Soluble HMW1C-like N-glycosyltransferases (NGTs) catalyze the glycosylation of Asn residues in proteins, a process fundamental for bacterial autoaggregation, adhesion and pathogenicity. In contrast, NGTs are two-domain enzymes that consists of an N-terminal all-α domain (AAD) and a C-terminal catalytic domain that adopts a GT-B fold, as shown for Actinobacillus pleuropneumoniae NGT (ApNGT). We focused on AaNGT, an inverting GT that catalyzes the transfer of Glc from UDP-Glc to Asn residues in the consensus sequence Asn-X-Ser/Thr. The heart-shaped structure of AaNGT, either complexed to UDP-Gal/UDP-2F-Glc or UDP-peptide, shows the N-terminal AAD domain and C-terminal GT-B fold catalytic domain, which is composed of an N- and C-Rossman fold subdomains.

A surface representation of the ternary complex reveals that UDP is partly buried and mainly recognized by the C-Rossmann fold subdomain while the peptide is more solvent exposed and tethered mostly by the N-Rossmann fold subdomain and the AAD domain. The UDP pyrophosphate of the ternary complex (AaNGT + UDP + peptide) exhibits more interactions than in the binary complexes, with Thr519, Asn520, and Gly521 backbones, and Ser277, Thr437, Lys440, and Asn520 side chains contributing to this. Additionally, interactions with Arg280 are observed in the ternary complex. Therefore, these more extensive interactions of UDP with the enzyme could explain the higher affinity of UDP compared to the sugar nucleotides. Multiple hydrogen bond interactions are observed at the peptide binding site in the ternary complex (AaNGT-peptide-UDP). The structural data demonstrate that the key residues involved in recognition of the peptide are Arg177, His214, and Asp215 from the AAD domain. In summary, the structural analysis shows that NGT shares two critical and conserved residues among NGTs, Arg177 and Asp215, in the AAD domain that recognize Thr and likely Ser at the +2 position of the Asn0-X+1-Ser/Thr+2 sequence motif. CH-π interactions between the peptide and the protein were also observed, in particular those involving Trp4+1 and the methylene group of Gln468 (AaNGT). The Asn at the acceptor position 0 in the sequence motif (Asn30) is located in front of the UDP pyrophosphate, although its side chain does not participate in interactions with any residue of AaNGT that could potentially serve as a catalytic base. Consequently, our ternary complex does not supply any evidence on how the Asn is glycosylated and thus no insights into the NGT catalytic mechanism could be inferred.

>[2x]MSRKKNPSVIQFEKAITEKNYEAACTELLDILNKIDTNFGDIEGIDFDYPQQLETLMQDRIVYFCTRMSNAITQLFCDPQFSLSESGANRFFVVQRWLNLIFASSPYINADHILQTYNCNPERDSIYDIYLEPNKNVLMKFAVLYLPESNVNLNLDTMWETDKNICGSLCFALQSPRFIGTPAAFSKRSTILQWFPAKLEQFHVLDDLPSNISHDVYMHCSYDTAENKHNVKKALNQVIRSHLLKCGWQDRQITQIGMRNGKPVMVVVLEHFHSSHSIYRTHSTSMIAAREQFYLIGLGNNAVDQAGRDVFDEFHEFDGSNILKKLAFLKEMCEKNDAAVLYMPSIGMDLATIFVSNARFAPIQVIALGHPATTHSEFIEYVIVEDDYVGSESCFSETLLRLPKDALPYVPSSLAPTDVQYVLRETPEVVNIGIAATTMKLNPYFLETLKTIRDRAKVKVHFHFALGQSIGITHPYVARFIRSYLGDDATAHPHSPYNRYLDILHNCDMMLNPFPFGNTNGIIDMVTLGLVGVCKTGPEVHEHIDEGLFKRLGLPEWLIADSVEDYIERAIRLAENHQERLALRRHIIENNGLKTLFSGDPSPMGKTLFAKLTEWRQTNGI;>FGNWTT[2x]> MKFSELWLREWVNPAIDSDALANQITMAGLEVDGVEPVAGSFNGVVVGEVVECAQHPNADKLRVTKVNVGGERLLDIVCGAPNCRQGLKVAVATIGAILPGDFKIKAAKLRGEPSEGMLCSFSELGISDDHSGIIELPADAPLGTDIREYLKLDDNTIEISVTPNRADCLGIIGVARDVAVLNKAPLQEPEMAPVTATISDTLPITVEAADACPRYLGRVVKGINVNAPTPLWMKEKLRRCGIRSIDAVVDVTNYVLLELGQPMHAFDKDRIDGGIVVRMAKEGETVVLLDGSEATLNADTLVIADHHKALGIAGIFWGEHSGVNGETQNVLLECAYFN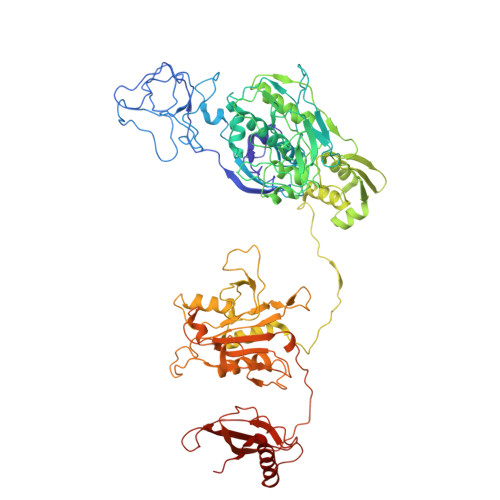PLSITGRARRHGLHTDASHRYERGVDPALQYKAIERATRLLLDICGGDAGPIIDVSNEATLPKRATITLRRSKLDRLIGHHIADEQVSDILRRLGCEVTEGQDEWKAVAPTWRFDMEIEEDLVEEVARVYGYNNIPDEPIQAGLIMGTHREADLSLKRVKTMLNDKGYQEVITYSFVDPKVQQLIHPGAEALLLPNPISVEMSAMRLSLWSGLLATVVYNQNRQQNRVRIFETGLRFVPDTQANLGIRQDLMLAGVICGNRYDEHWNLAKETVDFYDLKGDLEAVLDLTGKLGDIQFKAEMNPALHPGQSAAIYLKDERIGFIGVVHPELERKLDLNGRTLVFELEWNKLADRIVPQAREISRFPANRRDIAVVVAENVPAADILSECKKVGVNQVVGVNLFDVYRGKGVAEGYKSLAISLILQDTNRTLEEEEIAATVAKCVEALKERFQASLRD>MDLRDIDLNLLVVFNQLLLDRSVSTAGEKLGLTQPAVSNSLKRLRTALNDDLFLRTSKGMEPTPYALHLAEPVIYALNTLQTALTTRDSF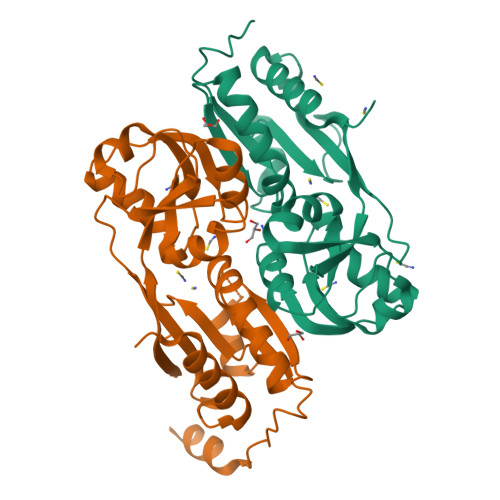DPFASTRTFNLAMTDIGEMSVMPPLMEALAQRAPHIQISTLRPNAGNLKEDMESGAVDLALGLLPELQTGFFQRRLFRHRYVCMFRKDHPSAKSPMSLKQFSELEHVGVVALNTGHGEVDGLLERAGIKRRMRLVVPHFIAIGPILHSTDLIATVPQRFAVRCEVPFGLTTSPHPAKLPDIAINLFWHAKYNRDPGNMWLRQLFVELFSEAHHHHHH[2x]>[4x]MKGFAMLSIGKVGWIEKEKPAPGPFDAIVRPLAVAPCTSDIHTVFEGAIGERHNMILGHEAVGEVVEVGSEVKDFKPGDRVVVPAITPDWRTSEVQRGYHQHSGGMLAGWKFSNVKDGVFGEFFHVNDADMNLAHLPKEIPLEAAVMIPDMMTTGFHGAELADIEMGSSVVVIGIGAVGLMGIAGAKLRGAGRIIGVGSRPICVEAAKFYGATDILNYKNGHI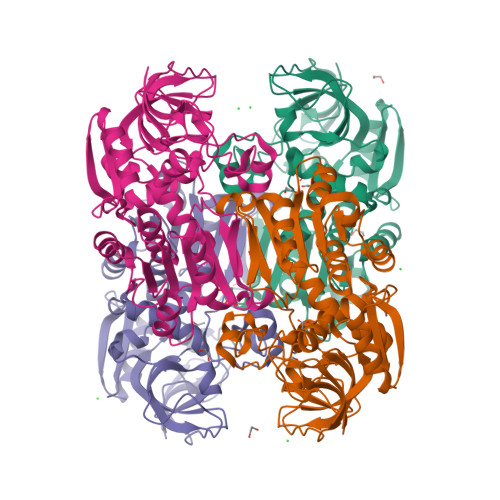VDQVMKLTNGKGVDRVIMAGGGSETLSQAVKMVKPGGIISNINYHGSGDALLIPRVEWGCGMAHKTIKGGLCPGGRLRMERLIDLVFYKRVDPSKLVTHVFRGFDNIEKAFMLMKDKPKDLIKPVVILA> MDVSRRQFFKICAGGMAGTTVAALGFAPKQALAQARNYKLLRAKEIRNTCTYCSVGCGLLMYSLGDGAKNAREAIYHIEGDPDHPVSRGALCPKGAGLLDYVNSENRLRYPEYRAPGSDKWQRISWEEAFSRIAKLMKADRDANFIEKNEQGVTVNRWLSTGMLCASGASNETGMLTQKFARSLGMLAVDNQARVUHGPTVASLAPTFGRGAMTNHWVDIKNANVVMVMGGNAAEAHPVGFRWAMEAKNNNDATLIVVDPRFTRTASVADIYAPIRSGTDITFLSGVLRYLIENNKINAEYVKHYTNASLLVRDDFAFEDGLFSGYDAEKRQYDKSSWNYQLDENGYAKRDETLTHPRCVWNLLKEHVSRYTPDVVENICGTPKADFLKVCEVLASTSAPDRTTTFLYALGWTQHTVGAQNIRTMAMIQLLLGNMGMAGGGVNALRGHSNIQGLTDLGLLSTSLPGYLTLPSEKQVDLQSYLEANTPKATLADQVNYWSNYPKFFVSLMKSFYGDAAQKENNWGYDWLPKWDQTYDVIKYFNMMDEGKVTGYFCQGFNPVASFPDKNKVVSCLSKLKYMVVIDPLVTETSTFWQNHGESNDVDPASIQTEVFRLPSTCFAEEDGSIANSGRWLQWHWKGQDAPGEARNDGEILAGIYHHLRELYQSEGGKGVEPLMKMSWNYKQPHEPQSDEVAKENNGYALED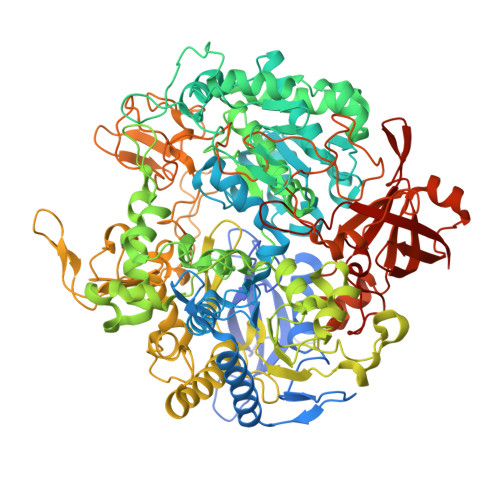LYDANGVLIAKKGQLLSSFAHLRDDGTTASSCWIYTGSWTEQGNQMANRDNSDPSGLGNTLGWAWAWPLNRRVLYNRASADINGKPWDPKRMLIQWNGSKWTGNDIPDFGNAAPGTPTGPFIMQPEGMGRLFAINKMAEGPFPEHYEPIETPLGTNPLHPNVVSNPVVRLYEQDALRMGKKEQFPYVGTTYRLTEHFHTWTKHALLNAIAQPEQFVEISETLAAAKGINNGDRVTVSSKRGFIRAVAVVTRRLKPLNVNGQQVETVGIPIHWGFEGVARKGYIANTLTPNVGDANSQTPEYKAFLVNIEKA>MSQHNEKNPHQHQSPLHDSSEAKPGMDSLAPEDGSHRPAAEPTPPGAQPTAPGSLKAPDTRNEKLNSLEDVRKGSENYALTTNQGVRIADDQNSLRAGSRGPTLLEDFILREKITHFDHERIPERIVHARGSAAHGYFQPYKSLSDITKADFLSDPNKITPVFVRFSTVQGGAGSADTVRDIRGFATKFYTEEGIFDLVGNNTPIFFIQDAHKFPDFVHAVKPEPHWAIPQGQAAHDTFWDYVSLQPETLHNVMWAMSDRGIPRSYRTMEGFGIHTFRLINAEGKATFVRFHWKPLAGKASLVWDEAQKLTGRDPDFHRRELWEAIEAGDFPEYELGFQLIPEEDEFKFDFDLLDPTKLIPEELVPVQRVGKMVLNRNPDNFFAENEQAAFHPGHIVPGLDFTNDPLLQGRLFSYTDTQISRLGGPNFHEIPINRPTCPYHNFQRDGMHRMGIDTNPANYEPNSINDNWPRETPPGPKRGGFESYQERVEGNKVRERSPSFGEYYSHPRLFWLSQTPFEQRHIVDGFSFELSKVVRPYIRERVVDQLAHIDLTLAQAVAKNLGIELTDDQLNITPPPDVNGLKKDPSLSLYAIPDGDVKGRVVAILLNDEVRSADLLAILKALKAKGVHAKLLYSRMGEVTADDGTVLPIAATFAGAPSLTVDAVIVPCGNIADIADNGDANYYLMEAYKHLKPIALAGDARKFKA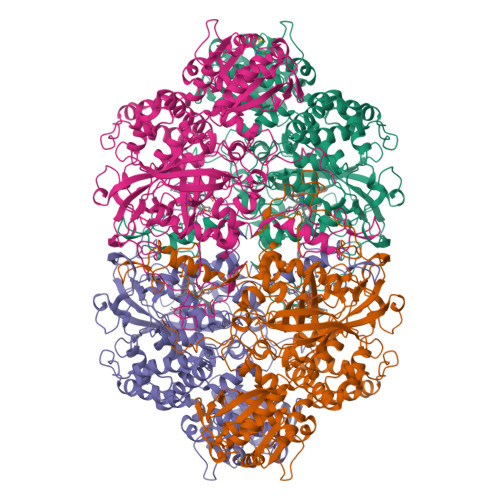TIKIADQGEEGIVEADSADGSFMDELLTLMAAHRVWSRIPKIDKIPA[4x]> MPLXXXXPPHGELQYLGQIQHILRCGVRKDDRTGTGTLSVFGMQARYSLRDEFPLLTTKRVFWKGVLEELLWFIKGSTNAKELSSKGVKIWDANGSRDFLDSLGFSTREEGDLGPVYGFQWR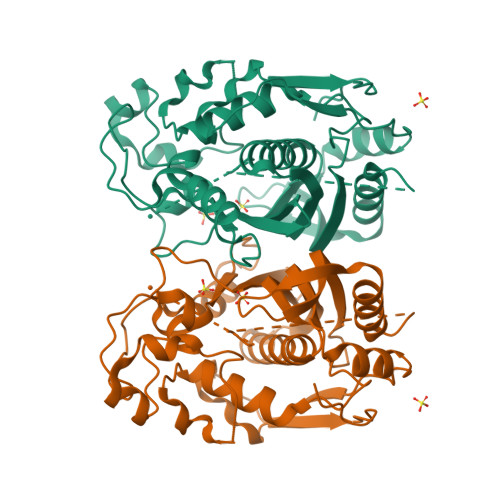HFGAEYRDMESDYSGQGVDQLQRVIDTIKTNPDDRRIIMCAWNPRDLPLMALPPCHALCQFYVVNSELSCQLYQRSGDMGLGVPFNIASYALLTYMIAHITGLKPGDFIHTLGDAHIYLNHIEPLKIQLQREPRPFPKLRILRKVEKIDDFKAEDFQIEGYNPHPTIKMEMAV>SLDHAKAEAELAINIKKATSPEETAPKRKHVRSCIVYTWDHKSSLSFWAGLKVQPILADEVQTFKALITIHKVLQE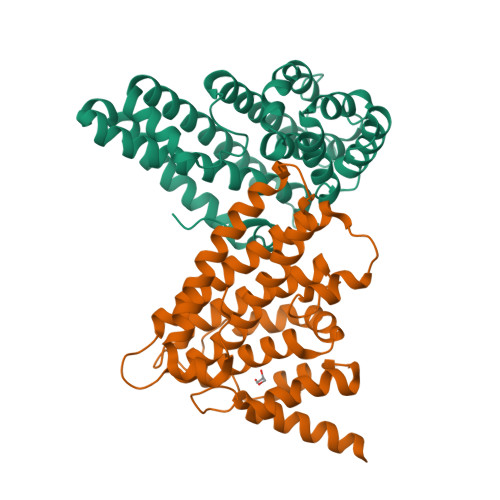GHPVTLREAMANRGWIDSLSRGMMGEGVRGYGPLIREYVHFLLAKLSFHKQHPEFNGTFEYEEYISLKAIHDPNEGYETITDLMTLQDKIDQFQKLIFSHFRHIGNNECRISALVPLVAESYGIYKFITSMLRAMHSSTGDNEALEPLRQRYDAQHYRLVKFYYECSNLRYLTSLITIPKL[2x]> GGCUUAUCAAGAGAGGGGGAGUGACUGGCGCGAAGACCCC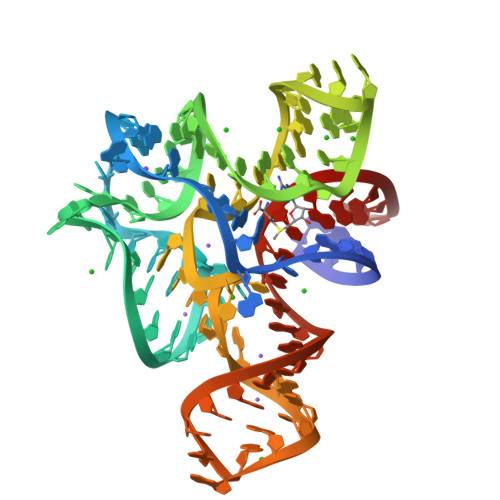CGGCAACCAGAAAUGGUGCCAAUUCCUGCAGCGGAAACGUUGAAAGAUGAGCCG Post-transcriptional exonucleolytic processing of U6 is directed by U6 biogenesis protein 1 (Usb1), a 3′–5′ exonuclease belonging to the 2H phosphodiesterase superfamily of enzymes. The highly conserved U6 snRNA coordinates magnesium ions in the active site that are required for splicing catalysis. We determined the 1.8 Å crystal structure of the catalytic domain of yUsb1, and a 1.4 Å co-crystal structure of hUsb1 bound to the substrate analog uridine 5′-monophosphate (5′ UMP). Here, we have demonstrated that two members of the 2H phosphodiesterase superfamily, yUsb1 and hUsb1, are mechanistically distinct, yet are involved in the same step of U6 biogenesis in their respective organisms.

Residues 107–115 could not be modeled in our structure and are presumed to be disordered. Despite low sequence identity (<20%), the structure of yUsb1 is strikingly homologous to that of human Usb111, with nearly superimposable active sites (root mean square deviation for H/S in active site=0.3 Å). NE2 of H231 is 2.8 Å from the sulfate ion, while H133 is farther away (4 Å). Our crystal structure reveals that residues 73–76 form the start of a β-strand and make several intramolecular contacts that are likely important for folding. In yeast, this position is a phenylalanine (F78) which cannot form an analogous hydrogen bond. Indeed, mutating F78 to alanine causes a slow growth phenotype in vivo and a >300-fold reduction in the rate of processing in vitro. Yeast Usb1 catalyzes two distinct chemical reactions: (1) exonucleolytic removal of a terminal uridine (“first step”) and (2) cyclic phosphodiesterase (CPDase) ring opening to leave a noncyclic phosphate (“second step”).

> GMSRFWRSFTYFEWRPTPAIHRQLQKIICKYKETFMKQEYTNPYQLVDFDPLFISHLGAPKPLHVSLTRSLLFETEEQRHVFIQEMRNGLRNNEITPFKLQICSYPKLYISERANTLYLGLPVSECPNKAQISPFKTIIAEALQKSGISNYQDLIVSRQNLHVSIAIASNPSKATLKRYQQLNETMGALLLLNNDFAYKLEFLVNSIYCDENRHSIRIPFN> KRQWALEDFEIGRPLGKGKFGNVYLAREKQSKFILALKVLFKAQLEKAGVEHQLRREVEIQSHLRHPNILRLYGYFHDATRVYLILEYAPLGTVYRELQKLSKFDEQRTATYITELANALSYCHSKRVIHRDIKPENLLLGSAGELKIAD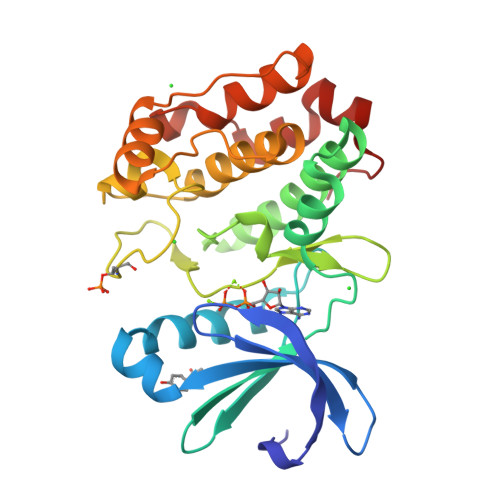FGWSVHAPSSRRTTLAGTLDYLPPEMIEGRMHDEKVDLWSLGVLCYEFLVGKPPFEANTYQETYKRISRVEFTFPDFVTEGARDLISRLLKHNPSQRPMLREVLEHPWITANSSKPSN> MPSEKEIL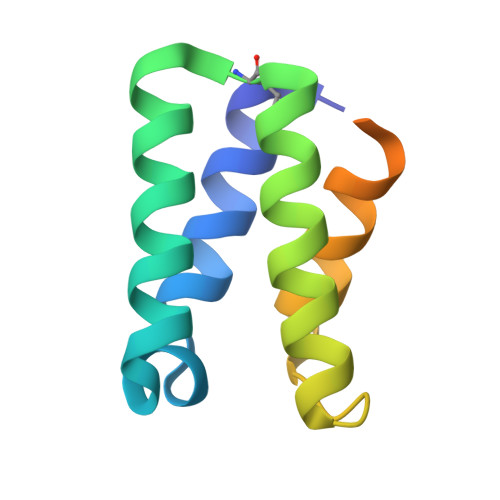DALSKVYSEQVIQADDYFRQAIFELASQLEKEGMSSLLATKIDSLINQYILTHQFDAPKSIFDLSRLVKTKASHYKGTAISAIMLGSFLSGGPK> EQSGISQTVIVGPW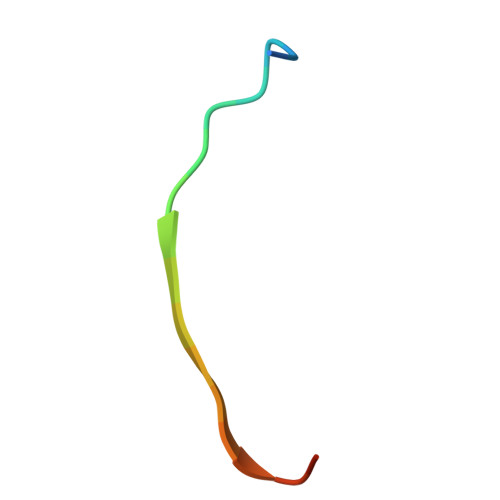GAKVS>MAHHHHHHMSKRAFNFCAGPAALPDAVLQRAQAELLDWRGKGLSVMEMSHRSDDYVAIASKAEQDLRDLLDIPSDYKVLFLQGGASQQFAEIPLNLLPEDGVADYIDTGIWSKKAIEEARRYGTVNVAASAKEYDYFAIPGQNEWTLTKDAAYVHYASNETIGGLEFDWIPETGDVPLVTDMSSDILSRPLDVSRFGLIYAGAQKNIGPSGLVVVIVREDLLGRARSVCPTMLNYKTAADNGSMYNTPATYSWYLSGLVFEWLKEQGGVTAMEQRNRAKKDLLYKTIDASDFYTNPIQPSARSWMNVPFRLADERLDKPFLEGAEARGLLNLKGHRSVGGMRASIY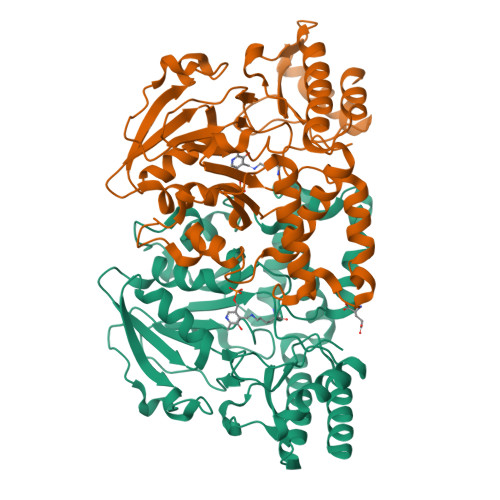NALGLDAVEALVAYMAEFEKEHG[2x]> MAAGFGRCCRVLRSISRFHWRSQHTKANRQREPGLGFSFEFTEQQKEFQATARKFAREEIIPVAAEYDKTGEYPVPLIRRAWELGLMNTHIPENCGGLGLGTFDACLISEELAYGCTGVQTAIEGNSLGQMPIIIAGNDQQKKKYLGRMTEEPLMCAYCVTEPGAGSDVAGIKTKAEKKGDEYIINGQKMWITNGGKANWYFLLARSDPDPKAPANKAFTGFIVEADTPGIQIGRKELNMGQRCSDTRGIVFEDVKVPKENVLIGDGAGFKVAMGAFDKTRPVVAAGAVGLAQRALDE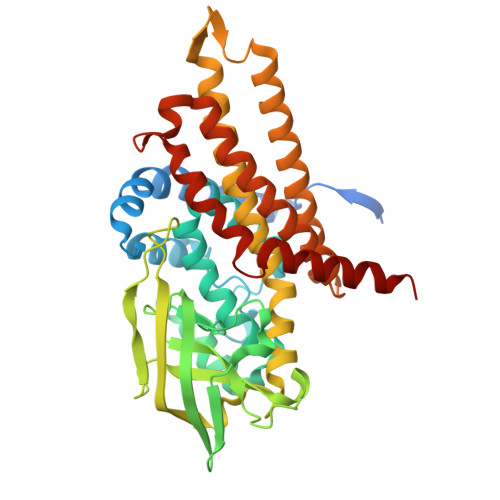ATKYALERKTFGKLLVEHQAISFMLAEMAMKVELARMSYQRAAWEVDSGRRNTYYASIAKAFAGDIANQLATDAVQILGGNGFNTEYPVEKLMRDAKIYQIYEGTSQIQRLIVAREHIDKYKN>SGFEFHGYARSGVIMNDSGASTKSGAYITPAGETGGAIGRLGNQADTYVEMNLEHKQTLDNGATTRFKVMVADGQTSYNDWTASTSDLNVRQAFVELGNLPTFAGPFKGSTLWAGKRFDRDNFDIHWIDSDVVFLAGTGGGIYDVKWNDGLRSNFSLYGRNFGDIDDSSNSVQNYILTMNHFAGPLQMMVSGLRAKDNDERKDSNGNLAKGDAANTGVHALLGLHNDSFYGLRDGSSKTALLYGHGLGAEVKGIGSDGALRPGADTWRIASYGTTPLSENWSVAPAMLAQRSKDRYADGDSYQWATFNLRLIQAINQNFALAYEGSYQYMDLKPEGYNDRQAVNGSFYKLTFAPTFKVGSI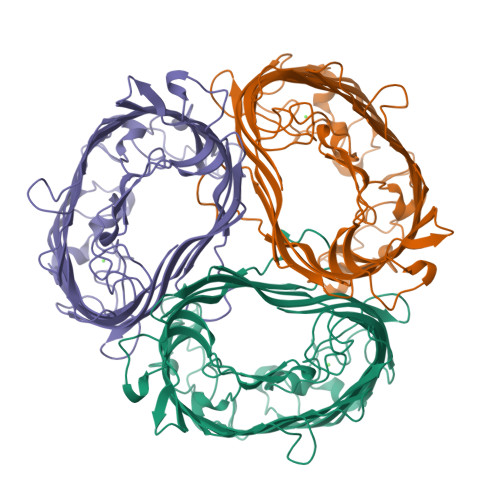GDFFSRPEIRFYTSWMDWSKKLNNYASDDALGSDGFNSGGEWSFGVQMETWF[3x]>[2x]KTPPVVFHWFPFIGSTISYGIDPYKFFFDCRAKYGDIFTFILLGKKTTVYLGTKGNDFILNGKLRDVCAEEVYSPLTTPVFGRHVVYDCPNAKLMEQKKFVKYGLTSDALRSYVPLITDEVESFVKNSPAFQGHKGVFDVCKTIAEITIYTASRSLQGKEVRSKFDSTFAELYHNLDMGFAPINFMLPWAPLPHNRKRDAAQRKLTETYM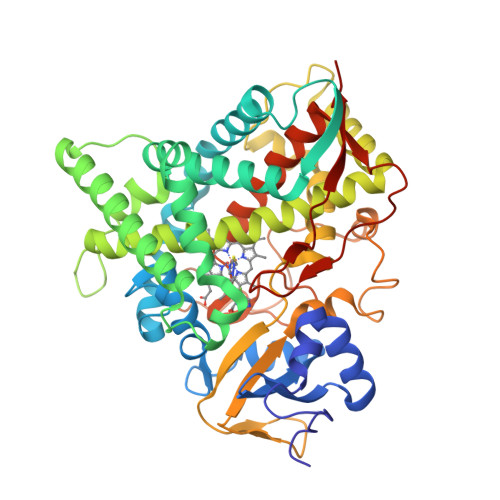EIIKARRQAGSKKDSEDMVWNLMSCVYKNGTPVPDEEIAHMMIALLMAGQHSSSSTASWIVLRLATRPDIMEELYQEQIRVLGSDLPPLTYDNLQKLDLHAKVIKETLRLHAPIHSIIRAVKNPMAVDGTSYVIPTSHNVLSSPGVTARSEEHFPNPLEWNPHRWDENIAASAEDDEKVDYGYGLVSKGTNSPYLPFGAGRHRCIGEQFAYLQLGTITAVLVRLFRFRNLPGVDGIPDTDYSSLFSKPLGRSFVEFEKRH1-(2-methyl-1H-indol-3-yl)-2-[(2R)-2-methylpiperidin-1-yl]ethan-1-one 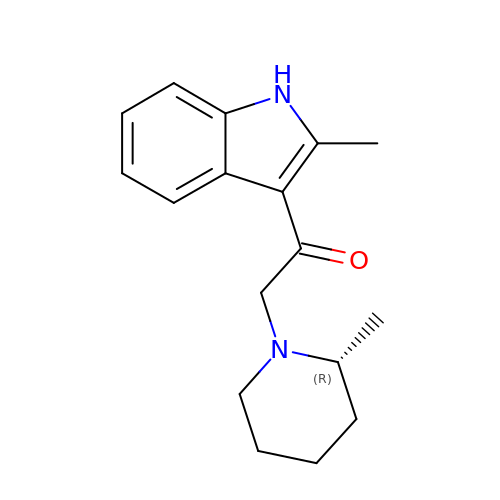| C17 H22 N2 O | VMIOFZFIOOEUFH-GFCCVEGCSA-N>MLVSVYLALLVACVGQAHSQANLMRLKSDLFNRSPMYPGPTKDDPLTVTLGFFLQDIVKVDSSTNEVDLVYYERQRWKLNSLMWDPNEYGNITDFRTSAADIWTPDITAASSTRPVQVLSPQIAVVTHDGSVMFSPAQRLSFMCDPTGVDSEEGVTCAVKFESWVYSGFEIDLKTDTDQVDLSSYYASSKYEILSATQTRQVQHYSCCPEPYIDVNLVVKFRERRAGNGFFRNLFDENLYFQGHHHHHH[5x]

Protein-engineering methods have been exploited to produce a surrogate system for the extracellular neurotransmitter-binding site of a heteromeric human ligand-gated ion channel, the glycine receptor. Acetylcholine-binding protein is a highly conserved ortholog of the pLGIC extracellular ligand-binding domain (ECD) with properties similar to nAChR. Mutations affecting key residues in the orthosteric agonist site at the α1(−)/β(+) interface affect the potency of both activation by glycine and inhibition by strychnine. We therefore set out to generate a high-fidelity surrogate of this α1(−)/β(+) orthosteric binding site using the 2α1:3β stoich­iometry [Fig. 1(a)] by exploiting protein-engineering methods and the thermal stability of acetylcholine-binding protein from Aplysia californica (AcAChBP). Ultimately, the highly stable AcAChBP framework has allowed us to introduce nine amino-acid substitutions that have resulted in a stable surrogate for a heteromeric neurotransmitter site that binds glycine.

Variant II therefore reverted back to Trp164, but with the inclusion of a G162E substitution. The residues now changed (Thr53, Gln74, Tyr110, Ile135 and Gly162) correspond to Phe72, Arg93, Ala146, Ser157 and Glu202 in the human GlyR-α1(−)/β(+) orthosteric site [Figs. 1(b) and 2]. Crystal structures of variant II with HEPES, tropisetron and strychnine revealed that the G162E substitution was accommodated with the structure essentially unperturbed compared with variant I, although now incorporating two charged residues (Arg74 and Glu162) to polarize the binding site such that the principal side is negatively charged and the complementary side is positive. The complex structure with HEPES showed this crystallization buffer component binding in two orientations in the orthosteric site in a similar fashion to that reported for LsAChBP.>SNAKLDQIRLYLDQKGAELAIFSDPVTINYLTGFFCDPHERQLFLFVYHDLAPVLFVPALEVARASQAISFPVFGYVDSENPWEKIKAVLPNTAAKTIYAEFDHLNVNKFHGLQTIFSGQFNNLTPYVQGMR[2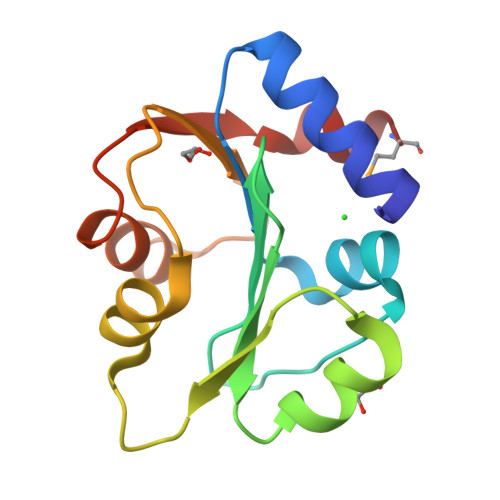x]In the heterocystous cyanobacterium Nostoc sp. PCC 7120, one such strategy is the use of an ArsR-SmtB transcriptional regulator RexT that senses H2O2 and upregulates expression of thioredoxin to maintain cellular redox homeostasis. Different from many other members of the ArsR-SmtB family which bind metal ions, RexT has been proposed to use disulfide bond formation as a trigger to bind and release DNA. Here, we present high-resolution crystal structures of RexT in the reduced and H2O2-treated states. These structures reveal that RexT showcases the ArsR-SmtB winged-helix-turn-helix fold and forms a vicinal disulfide bond to orchestrate a response to H2O2. Each protomer of RexT has an α1-α2-α3-α4-β1-β2-α5a/b architecture.

Second, this SeMet structure was used as a model for the molecular replacement to determine a higher resolution structure of native RexT to 1.95-Å resolution. The asymmetric unit of the RexT crystal structure contains a homodimer of RexT, which is consistent with the oligomeric state observed in solution using size-exclusion chromatography. The dimer interface of RexT is formed by a coiled-coil interaction between the α1 helices (residues 13–22) and between the α5b helices (residues 91–96) of each protomer. The buried interface area is 707.6 Å2, ~11.5-percent of the total surface area of each protomer. The location of the Cys105 residue, which is only modeled in chain B of the determined structure is located ~20 Å away from both Cys40 and Cys41. Similarly, in both monomeric units of the reduced RexT structure, the mainchain amide of the corresponding Cys41 interacts with a molecule, which is best modeled as a chloride anion from the crystallization buffer. In the dimeric structure of RexT, the wHTH region shows an overall positive electrostatic potential and appears well-poised to interact with DNA.

>[2x]GSMRFLYHPDRKDISLPGVLYALGDPARLEIVRLLASKGEQCCAEFDFAIAKSTMSNHFKILRESGVVLTRKEGTQHINRLRREDLETLFPGLLDAVLRSAQPLLTCQQSAIVK> VGSLNCIVAVSQNMGIGKNGDLPWPPLRNEFRYFQRMTTTSSVEGKQNLVIMGKKTWFSIPEKNRPLKGRINLVLSRELKEPP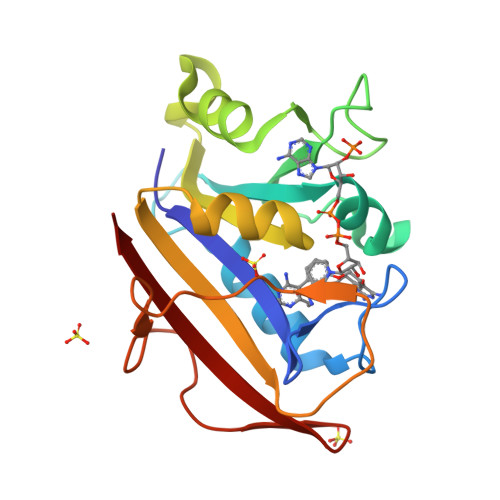QGAHFLSRSLDDALKLTEQPELANKVDMVWIVGGSSVYKEAMNHPGHLKLFVTRIMQDFESDTFFPEIDLEKYKLLPEYPGVLSDVQEEKGIKYKFEVYEKND>MESEQLFHRGYYRNSYNSITSASSDEELLDGAGVIMDFQTSEDDNLLDGDTAVGTHYTMTNGGSINSSTHLLDLLDEPIPGVGTYDDFHTIDWVREKCKDRERHRRINSKKKESAWEMTKSLYDAWSGWLVVTLTGLASGALAGLIDIAADWMTDLKEGICLSALWYNHEQCCWGSNETTFEERDKCPQWKTWAELIIGQAEGPGSYIMNYIMYIFWALSFAFLAVSLVKVFAPYACGSGIPEIKTILSGFIIRGYLGKWTLMIKTITLVLAVASGLSLGKEGPLVHVACCCGNIFSYLFPKYSTNEAKKREVLSAASAAGVSVAFGAPIGGVLFSLEEVSYYFPLKTLWRSFFAALVAAFVLRSINPFGNSRLVLFYVEYHTPWYLFELFPFILLGVFGGLWGAFFIRANIAWCRRRKSTKFGKYPVLEVIIVAAITAVIAFPNPYTRLNTSELIKELFTDCGPLESSSLCDYRNDMNASKIVDDIPDRPAGIGVYSAIWQLCLALIFKIIMTVFTFGIKVPSGLFIPSMAIGAIAGRIVGIAVEQLAYYHHDWFIFKEWCEVGADCITPGLYAMVGAAACLGGVTRMTVSLVVIVFELTGGLEYIVPLMAAVMTSKWVGDAFGREGIYEAHIRLNGYPFLDAKEEFTHTTLAADVMRPRRNDPPLAVLTQDNMTVDDIENMINETSYNGFPVIMSKESQRLVGFALRRDLTIAIESARKKQEGIVGSSRVCFAQHTPSLPAESPRPLKLRSILDMSPFTVTDHTPMEIVVDIFRKLGLRQCLVTHNGRLLGIITKKDILRHMAQTANQDPASIMFN[2x];>[2x]MKLLSLVAVVGCLLVPPAEANKSSEDIRCKCICPPYRNISGHIYNQNVSQKDCNCLHVVEPMPVPGHDVEAYCLLCECRYEERSTTTIKVIIVIYLSVVGALLLYMAFLMLVDPLIRKPDAYTEQLHNEEENEDARSMAAAAASLGGPRANTVLERVEGAQQRWKLQVQEQRKTVFDRHKMLS

Five members of the CLC family of Cl− channels and Cl−/H+ exchangers, ClC-3, ClC-4, ClC-5, ClC-6 and ClC-7, have critical roles in endosomes and lysosomes, catalyzing the exchange of two Cl− ions for one H+ ion2,10–12. We recently found that the ClC-3, ClC-4 and ClC-5 clade of endosomal CLC transporters requires the accessory β-subunit TMEM9, which we refer to as T9A or its closely related homolog TMEM9B (T9B) for proper activity in cells and animals. To resolve the mechanism by which T9A and T9B regulate the activity of ClC-3, ClC-4 and ClC-5, we determined structures of ClC-3 alone and in complex with T9A, finding that T9A occludes the Cl− ion pathway and that inhibition requires the endolysosomal signaling lipid phosphatidylinositol 3,5-bisphosphate (PtdIns(3,5)P2). Each ClC-3 protomer comprises a cytosolic N-terminal domain (NTD), a transmembrane domain (TMD) and a cytosolic domain (CD).

We identified a two-fold symmetric class in which the luminal domain (LD), TMD and CD of both T9A protomers are resolved, which we call ClC-3/T9A. To distinguish this fourth class from the structure of ClC-3 determined in the absence of T9A, we call this class ClC-3/noT9A. Because of its completeness, we focus our discussion primarily on ClC-3/T9A, which achieved a resolution of 2.9 Å with C2 symmetry imposed. In ClC-3/T9A, T9A wraps around ClC-3, interacting with the luminal, transmembrane and cytosolic faces of the ClC-3 TMD. The T9A LD interacts primarily with the ClC-3 helix B insertion, forming both polar and nonpolar interactions, including the embedding of F181 of ClC-3 into a hydrophobic groove on T9A and an extended π-stacking interaction between R28 and R83 of T9A with W174 of ClC-3. The single membrane-spanning helix of T9A, helix H3, extends along the periphery of the ClC-3 TMD, forming interactions with helices B, C, E and I of ClC-3. The T9A CD consists of the H4 helix that extends along the cytosolic face of the ClC-3 TMD and four residues at the extreme C terminus, which we define as the CTD. Whereas both entrances of the Cl− ion pathway are solvent accessible in the absence of T9A, the CDs of T9A constrict the cytosolic entrances to the Cl− pathway in ClC-3/T9A to a minimum radius of 0.9 Å, which is too narrow to accommodate a Cl− ion. We, therefore, assign ClC-3/T9A as an inhibited state, with the T9A CD forming the gate. In ClC-3/T9A, PtdIns(3,5)P2 interacts with both ClC-3 and the T9A CD. Thus, PtdIns(3,5)P2 appears to serve as a bridge between ClC-3 and the T9A CD, raising the possibility that PtdIns(3,5)P2 influences the equilibrium between the bound and unbound states of the T9A CD to regulate ClC-3 activity.>MSVVSQVILQADDQLRYPTSGELKGIQAFLTTGAQRIRIAETLAENEKKIVDQAQKQLFKKHPEYRAPGGNAYGQRQYNQCLRDYGWYLRLVTYGVLAGNKEPIETTGLIGVKEMYNSLNVPVPGMVDAVTVLKDAALGLLSAEDANETAPYFDYIIQFMSHHHHHH[3x];>[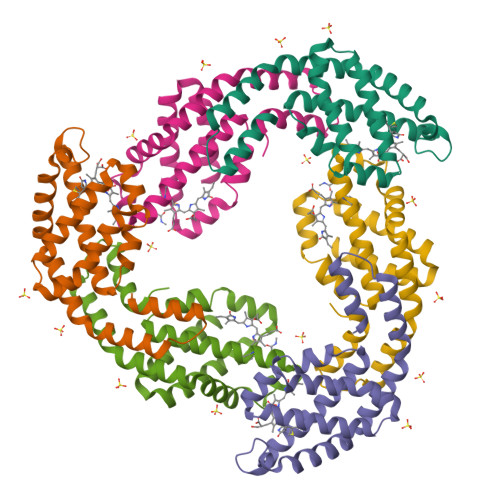3x]MQDAITAVINSADVQGKYLDGAAMDKLKSYFASGELRVRAASVISANAATIVKEAVAKSLLYSDVTRPGGNMYTTRRYAACIRDLDYYLRYATYAMLAGDASILDERVLNGLKETYNSLGVPISSTVQAIQAIKEVTASLVGADAGKEMGVYLDYICSGLS>IPAGIIPTGNVLSTIEVCIFFCIFDFFKQIRSDDNSLYSAQFDILLGTYCNTLNFVRFLELGLSVACICTKFPELAYVRDGVIQFEVQQPMIARDGPHPVDQPVHNYMVKRIHKRSLSAAFAIASEALSLLSNTYVAATEIDSSLRIRAIQQMARNLRTVSDSFERGTADQLLGVLLEKAPPLSLLSPINKFQPEGHLNRVARAALLSDLKRRVCADMFFMTRHAREPRLISAYLSDMVSCTQPSVMVSRITHTNTRGRQVDGVLVTTATLKRQLLQGILQIDDTAADVPVTYGEMVLQGTNLVTALVMGKAVRGMDDVARHLLDITDPNTLNIPSIPPQSNSDSTTAGLPVNARVPADLVIVGDKLVFLEALERRVYQATRVAYPLIGNIDITFIMPMGVFQANSMDRYTRHAGDFSTVSEQDPRQFPPQGIFFYNKDGILTQLTLRDAMGTICHSSLLDVEATLVALRQQHLDRQCYFGVYVAEGTEDTLDVQMGRFMETWADMMPHHPHWVNEHLTILQFIAPSNPRLRFELNPAFDFFVAPGDVDLPGPQRPPEAMPTVNATLRIINGNIPVPLCPISFRDCRGTQLGLGRHTMTPATIKAVKDTFEDRAYPTIFYMLEAVIHGNERNFCALLRLLTQCIRGYWEQSHRVAFVNNFHMLMYITTYLGNGELPEVCINIYRDLLQHVRALRQTITDFTIQGEGHNGETSEALNNILTDDTFIAPILWDCDALIYRDEAARDRLPAIRVSGRNGYQALHFVDMAGHNFQRRDNVLIHGRPVRGDTGQAIPITPHHDREWGILSKIYYYIVIPAFSRGSCCTMGVRYDRLYPALQAVIVPEIPADEEAPTTPEDPRHPLHAHQLVPNSLNVYFHNAHLTVDGDALLTLQELMGDMAERTTAILVSSAPDAGAATATTRNMRIYDGALYHGLIMMAYQAYDETIATGTFFYPVPVNPLFACPEHLASLRGMTNARRVLAKMVPPIPPFLGANHHATIRQPVAYHVTHSKSDFNTLTYSLLGGYFKFTPISLTHQLRTGFHPGIAFTVVRQDRFATEQLLYAERASESYFVGQIQVHHHDAIGGVNFTLTQPRAHVDLGVGYTAVCATAALRCPLTDMGNTAQNLFFSRGGVPMLHDNVTESLRRITASGGRLNPTEPLPIFGGLRPATSAGIARGQASVCEFVAMPVSTDLQYFRTACNPRGRASGMLYMGDRDADIEAIMFDHTQSDVAYTDRATLNPWASQKHSYGDRLYNGTYNLTGASPIYSPCFKFFTPAEVNTNCNTLDRLLMEAKAVASQSSTDTEYQFKRPPGSTEMTQDPCGLFQEAYPPLCSSDAAMLRTAHAGETGADEVHLAQYLIRDASPLRGCLPL[5x];> AMPFEIEVLLPGELSPAETSALQKCEGKIITFSTLRHRASLVDIALSSYYINGAPPDTLSLLEAYRMRFAAVITRVIPGKLLAHAIGVGTPTPGLFIQNTSPVDLCNGDYICLLPPVYGSADSIRLDSVGLEIVFPLTIPQTLMREIIAKVVARAVEDLNLMFSINEGCLLILALIPRLLALLIPRLLALVTREAAQLIHPEAPMLMLPIYETISSWISTSSRLGDTLGTRAILRVCVFDGPSTVHPGDRTAVIQV;> AMPFEIEVLLPGEISPAETSALQKCEGKIITFSTLRHRASLVDIALSSYYINGAPPDTLSLLEAYRMRFAAVITRVIPGKLLAHAIGVGTPTPGLFIQNTSPVDLCNGDYICLLPPVFGSADEIRLDSVGLEIVFPLTIPQTLMREIIAKVVARAVERTAADVICYNGRRYELETNLQHRDGSDAAIRTLVLNLMFSINEGTTLILTLITRLLRFPIYEAISSWISTSSRLGDTLGTRAILRVCVFDGPSTVHPGDRTAVIQV;> FKSTTQLIQQVSLTDFFRPDIEHAGSTVLILRHPTDLPALARHRAPPGRQTERLAEAWGQLLEASRAYVTSLSFIAACRAEEYTDKQAAEANRTAIVSAY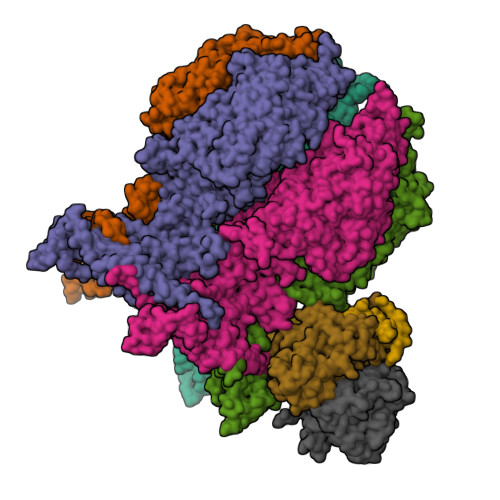GCSRMGARLIRFSECLRAMVQCHVFPHRFISFFGSLLEYTIQDNLCNITAVAKGPQEAARTDKTSTRRVTANIPACVFWDVDKDLHLSADGLKHVFLVFVYTQRRQREGVRLHLALSQLNEQCFGRGIGFLLGARICMYAAYTLIGTIPSESVRYTRRMERFGGYNVPTIWLEGVVWGGTNTWNEC> MFGYFYNSSFRRYATLMGDLFSNIQIKRQLESGDKFIRVPITYASKEHFMMKLNKWTSI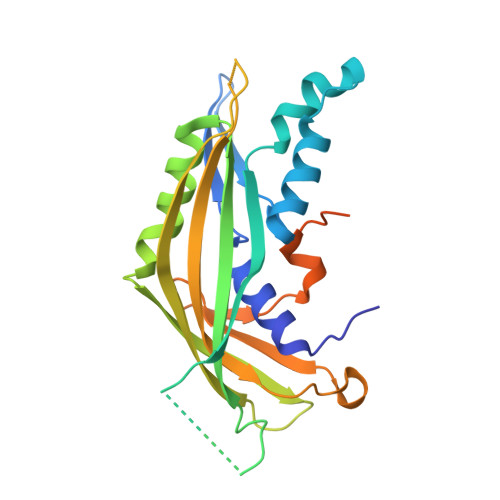NSQEDVAKVETILPRINLHLVDFSYNAPFKTNILNQNLLQKGATSVVSQYNPSPIKMIYELSIFTRYEDDMFQIVEQILPYFQPHFNTTMYEQFGNDIPFKRDIKIVLMSAAIDEAIDGDNLSRRRIEWSLTFEVNGWMYPPVDDAEGLIRTTYTDFHANTRDLPDGEGVFESVDSEVVPRDIDPEDWDGTVKQTFTSNVNRPTPPEPPGPRT>[2x]GSMPNFGFHIAPTHPVAGRLTYDSKKLSENILKQQSDERVFSRAQEQKRLSEGDVVGGAPCCKAIHITLGFDGTNN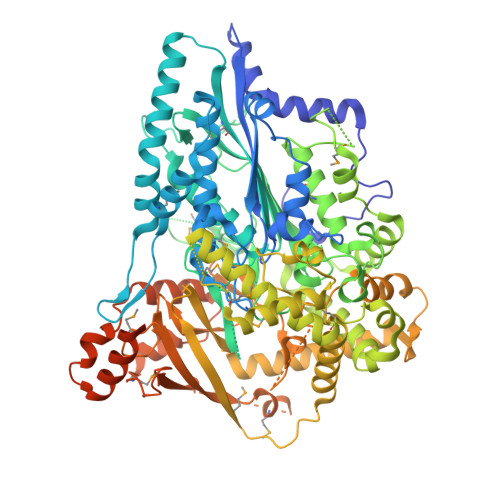NDKADGSSVSPSCSNVARLIHASIGSGDDINSRGIFKYYCPGVGTVFPDIKEFTPSNMGLIGAEGGENRINWGLVQLVDALFYTLLKSRLKLNDVQGLVEEMSTNWTVSTLTGGLLENGEKKRRAALEPKLKELEEKLRQRQNSGQKPHILAMRLYIYGFSRGAAEARAFANWLQELTRVSDADGRVEYRFAGLPISIEFLGLFDTVAAVGLADSAPFAAGHMDWADDTMRLPDEALSQCLPTILPEDCSFLKRCVHLVSCHEQRASFPLDSIRRRDMDANGRRTGPSCYRKWTVEYAYPGVHSDVGGGYGVGNQGKAVGGSEFLLSQIALQHMYAEAFEAGAPLQVPAPAVHPDFHEEWRVMVPKIEAEFSVSEELATRFNAWQAQAKAGPLEEVIRRETALITAWRIDRYAGGLRNKAFFANVPPDMPEAQQKAWEALHKRRSREYAAAQQGEPLPPMSAAEQAEWDRNVALIGGEDQLRDLRVEKQFDPPLDQRQLLGAAAEFAHDYKGDWGVLDDGMTVGGVIDLLLGGTVFLINEEDEAEEYSQIHRDGSARYHQLFSAPDRVAPGQEKLVALFDEQVHDSRAWFMNTSAIGPREPFTDYFRYRLVHFDNESNKRLSVLATAGRVVGVGVMLASVGLSVKRRDPRMLLGLFLPSLARPLLSGKVGLPEISAFDPLTGIALPMVGGAALDNLRAFTREPGDKVEQIGQLPPPPPLAVAAVQSPALQQVLLAQQTVEALKARDLGSLAGLVAKAELTQAPAAATPAWLAEAKQALQDMGTEQAQPPGPGSAPGWLKRGKDLMESL>TSELRICRINKESGPCTGGEELYLLCDKVQKEDISVVFSTASWEGRADFSQADVHRQIAIVFKTPPYEDLEISEPVTVNVFLQRLTDGVCSEPLPFTYLPR[3x];>ASNLKISRMDKTAGSVRGGDEVYLLCDKVQKDDIEVRFYEDDENGWQAFGDFSPTDVHKQYAIVFRTPPYHKMKIERPVTVFLQLKRKRGGDVSDSKQFTYYPV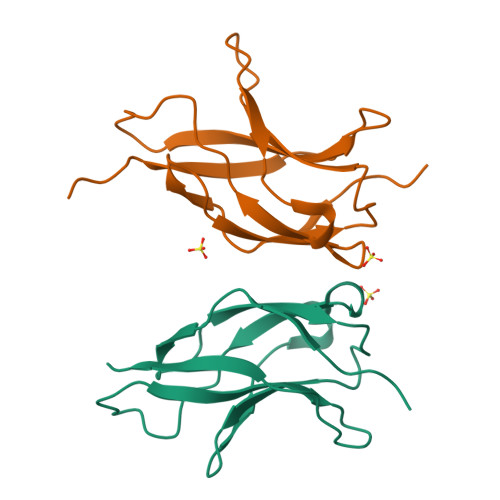VED[3x]4-(1H-IMIDAZOL-1-YL)PHENOL | C9 H8 N2 O | 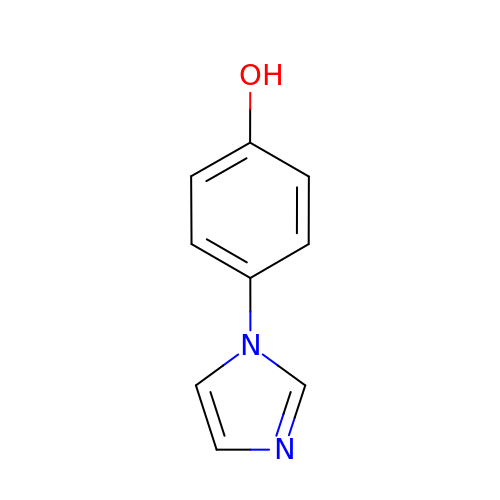CYKCUAPYWQDIKR-UHFFFAOYSA-N>[2x]EPTCNTPSNRACWSDGFDINTDYEVSTPDTGVTQSYVFNLTEVDNWMGPDGVVKEKVMLINGNIMGPNIVANWGDTVEVTVINNLVTNGTSIHWHGIHQKDTNLHDGANGVTECPIPPKGGQRTYRWRARQYGTSWYHSHFSAQYGNGVVGTIQINGPASLPYDIDLGVFPITDYYYRAADDLVHFTQNNAPPFSDNVLINGTAVNPNTGEGQYANVTLTPGKRHRLRILNTSTENHFQVSLVNHTMTVIAADMVPVNAMTVDSL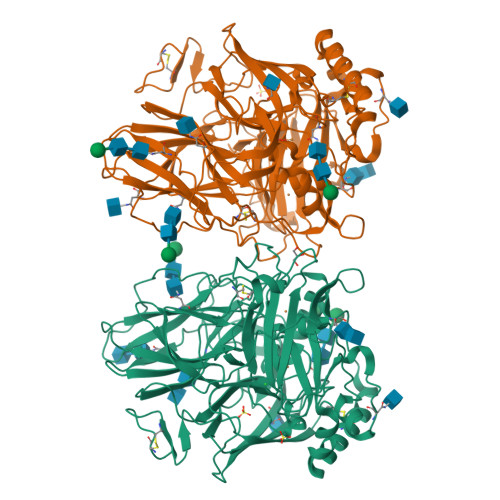FLAVGQRYDVVIDASRAPDNYWFNVTFGGQAACGGSLNPHPAAIFHYAGAPGGLPTDEGTPPVDHQCLDTLDVRPVVPRSVPVNSFVKRPDNTLPVALDLTGTPLFVWKVNGSDINVDWGKPIIDYILTGNTSYPVSDNIVQVDAVDQWTYWLIENDPEGPFSLPHPMHLHGHDFLVLGRSPDVPAASQQRFVFDPAVDLARLNGDNPPRRDTTMLPAGGWLLLAFRTDNPGAWLFHCHIAWHVSGGLSVDFLERPADLRQRISQEDEDDFNRVCDEWRAYWPTNPYPKIDSGA> GSMDYDFKVKLSSERERVEDLFEYEGCKVGRGTYGHVYKAKRKDGKDDKDYALKQIEGTGI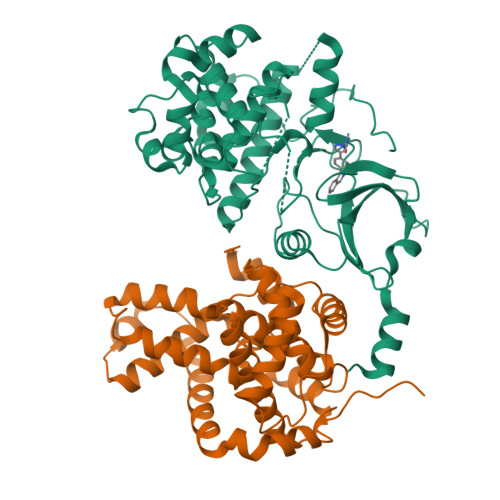SMSACREIALLRELKHPNVISLQKVFLSHADRKVWLLFDYAEHDLWHIIKFHRASKANKKPVQLPRGMVKSLLYQILDGIHYLHANWVLHRDLKPANILVMGEGPERGRVKIADMGFARLFNSPLKPLADLDPVVVTFWYRAPELLLGARHYTKAIDIWAIGCIFAELLTSEPIFHCRQEDIKTSNPYHHDQLDRIFNVMGFPADKDWEDIKKMPEHSTLMKDFRRNTYTNCSLIKYMEKHKVKPDSKAFHLLQKLLTMDPIKRITSEQAMQDPYFLEDPLPTSDVFAGCQIPYPKREFLTEEEPDDKGDKKNQQQQQGNNHTNGTGHPGNQDSSHTQGPPLKK;> GSMAGNFWQSSHYLQWILDKQDLLKERQKDLKFLSEEEYWKLQIFFTNVIQALGEHLKLRQQVIATATVYFKRFYARYSLKSIDPVLMAPTCVFLASKVEEFGVVSNTRLIAAATSVLKTRFSYAFPKEFPYRMNHILECEFYLLELMDCCLIVYHPYRPLLQYVQDMGQEDMLLPLAWRIVNDTYRTDLCLLYPPFMIALACLHVACVVQQKDARQWFAELSVDMEKILEIIRVILKLYEQWKNFDERKEMATILSKMPKPKPPPNSEGEQGPNGSQNSSYSQS N-[(2R,3S)-2-(4-chlorophenyl)-1-(1,4-dimethyl-2-oxo-1,2-dihydroquinolin-7-yl)-6-oxopiperidin-3-yl]-2-methylpropane-1-sulfonamide 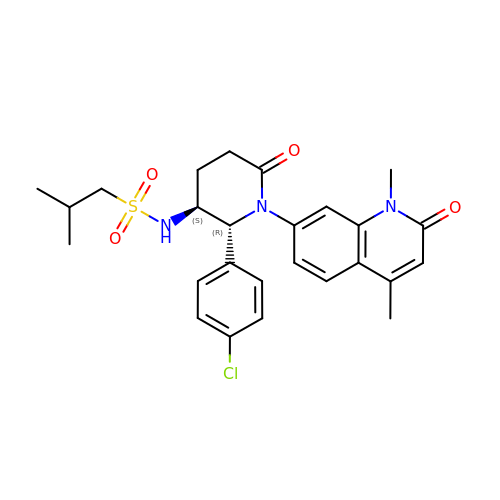| C26 H30 Cl N3 O4 S | LVDRREOUMKACNJ-BKMJKUGQSA-N>GKNPVESVSVEFEAKSARDGAWYDVAAFLSHRLFESGDPEVRVRFSGFGAEEDEWINVRKCVRQRSLPCEATECVAVLPGDLILCFQEGKDQALYYDAHVLDAQRRRHDVGGCRCRFLVRYDHDSSEEIVPLRKVCRRPE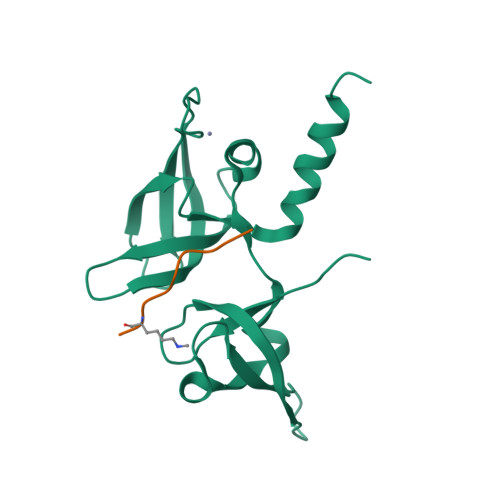TDYRLQILHAARAAATN[2x];>ARTKQTARKS[2x]>MHHHHHHSSGRENLYFQGTLSALAVDLGGTNLRVAIVSMKGEIVKKYTQFNPKTYEERINLILQMCVEAAAEAVKLNCRILGVGISTGGRVNPREGIVLHSTKLIQEWNSVDLRTPLSDTLHLPVWVDNDGNCAALAERKFGQGKGLENFVTLITGTGIGGGIIHQHELIHGSSFCAAELGHLVVSLDGPDCSCGSHGCIEAYASGMALQREAKKLHDEDLLLVEGMSVPKDEAVGALHLIQAAKLGNAKAQSILRTAGTALGLGVVNILHTMNPSLVILSGVLASHYIHIVKD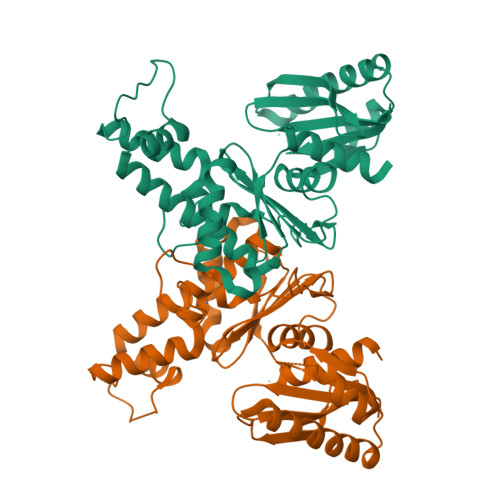VIRQQALSSVQDVDVVVSDLVDPALLGAASMVLDYTTRR[3x]The African swine fever virus (ASFV) type II topoisomerase (Topo II), pP1192R, is the only known Topo II expressed by mammalian viruses and is essential for ASFV replication in the host cytoplasm. In ASFV, a functional viral Topo II pP1192R has been identified, encoded by a viral gene conserved in ASFV strains, P1192R. pP1192R is detectable at an intermediate to late stage of ASFV infection, mainly within the cytoplasmic virus factory, and has been confirmed to be important for ASFV replication. Topo IIAs exhibit a 2-fold symmetry and comprise two functional domains: an ATPase domain and a DNA binding/cleavage domain. The mechanism of enzymatic action involves the opening and closing of three gate-like dimeric interfaces, which are called the N-, DNA- and C-gate, respectively, upon ATP binding and hydrolysis and DNA cleavage that introduces a double-strand break in the DNA (G-segment) trapped in the DNA-gate for transport of another DNA strand (T-segment).

To capture the intact structure of full-length pP1192R, the protein sample was then analyzed by single-particle cryo-EM. After collecting and processing 2134 cryo-EM images, two types of particles, referred to as State 1 and State 2, were identified and reconstructed to the overall resolution of 2.77 and 2.98 Å with 131 161 and 78 195 particles, respectively. The electron density was only observable for the DNA binding/cleavage domain in both states, while the electron density of the N-terminal ATPase domain was absent. Following the process of atomic model building based on the EM density map, the apo structure of the pP1192R DNA binding/cleavage domain was well resolved in both states, with the C-terminus of the protein (C-gate) adopting distinct conformations, accordingly described as ‘open’ (State 1) and ‘closed’ (State 2). These apo structures can be traced for 779 residues, ranging from D416 to H1192, except for the region containing residues G471-N501. The other typical domains of the DNA binding/cleavage core characterized in Topo IIAs, that is, the metal-binding topoisomerase/primase (TOPRIM) domain, the catalytic tyrosine (Y800 in pP1192R)-containing winged helix domain (WHD), the Tower domain, and the coiled-coil helices, are well illustrated in the two pP1192R apo structures. In the closed state, an extra dimeric interface, the C-gate, was formed by the interaction between the coiled-coil helices of two protomers, which retains a distance of ∼16 Å in the open state. No significant conformational changes were observed in the DNA-binding groove when comparing the two apo states, while the coiled-coil helices underwent a distinct conformational rearrangement, presenting the dynamic cycling of the C-gate between open to closed. The coiled-coil regions (from A' α14 to A' α18) of each protomer move towards one another in the closed state, with the furthest end moving a distance of ∼13.4 Å and a reorientation of ∼12° relative to the open state.

>[2x]METFEISDFKEHAKKKSMWAGALNKVTISGLMGVFTEDEDLMALPIHRDHCPALLKIFDELIVNATDHERACHNKTKKVTYIKISFDKGVFSCENDGPGIPIVKHEQASLIAKRDVYVPEVASCYFLAGTNINKAKDCIKGGTNGVGLKLAMVHSQWAILTTADGSQKYVQHINQRLDNIEPPTITPSREMFTRIELMPVYQELGYAQPLSETEQADLSAWIYLRACQCAAYVGKGTTIYYNDKPCSTSSVMALAKMYTLVTAPNSTIYTATIKADAKPYSLHPLQVAAVVSPKFKKFEHVSIINGVNCVKGEHVTFLKKAINEMVVKKFQQTIKDKNRKTTLRDSCSNIFVVIVGSIPGIEWTGQRKDELSIAENVFKTHYSIPSSFLTSMTRSIVDILLQSISKKDNHKQIDVDKYTRARNAGGKKAQDCMLLAAEGDSALSLLRAGLTLGKSNPSGPSFDFCGMISLGGVIMNACKKVTNITTDSGETIMVRNEQLTNNKVLQGIVQVLGLDFNCHYKTQEERAKLRYGCIVACVDQDLDGCGKILGLLLAYFHLFWPQLIVHGFVKRLLTPLIRVYEKGNTVPVEFYYEQEFDAWAKKQTSLANHTVKYYKGLAAHDTHEVKSMFKHFDKMVYTFTLDDSAKELFHIYFGGESELRKRELCTGVVPLTETQTQSIHSVRRIPCSLHLQVDTKAYKLDAIERQIPNFLDGMTRARRKILAGGLKCFASNNRERKVFQFGGYVADHMFYHHGDMSLNTSIIKAAQYYPGSSHLYPVFIGIGSFGSRHLGGKDAGSPRYISVQLASEFIKTMFPTEDSWLLPYVFEDGQRAEPEYYVPVLPLAIMEYGANPSEGWKYTTWARQLEDILALVRAYVDKNNPKHELLHYAIDHKITVLPLRPSNYNFKGHLKRFGQYYYSYGTYVVSEQRNMITITELPLRVPTVAYIESIKKSSNRMAFIEEIVDYSSSETIEILVKLKPNSLSRIMEEFKETEEQNSIENFLRLRNCLHSHLNFVKPKGGIIEFNSYYEILYAWLPYRRDLYQKRLMRERAVLKLRLIMETAIVRYINESADLNLSHYEDEKEAGRILSEHGFPPLNQSLITSPEFATIEELNQKALQGCYTYILSLQARELLIAAKTRRVEKIKKMQARLDKVEQLLQESPFPGASVWLEEIDAVEKAIIKGRNTQWKFH>[2x]ASSVEYDDSV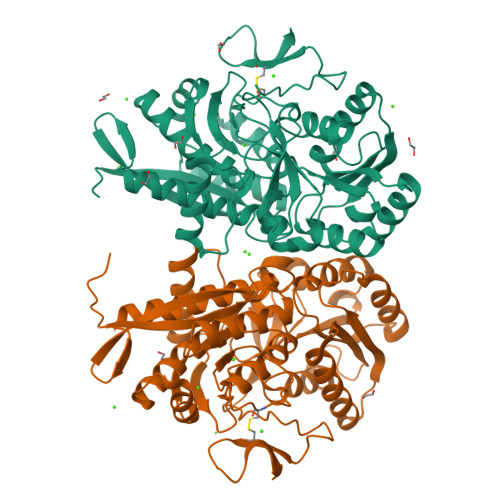TVGILHSLTGTMAISESTLVDTEKMAIDEINAAGGVEVDGKKYKIEYIVEDGASDWPTFAEKSKKLIDQDKVPVVFGGWTSASRKAMLPVYESKEAFLYYPIQYEGQECSKNIFYTGATPNQQSEPATSYMFEKSPAAGKPFYLVGSDYVFPRTSNTITKEQVKSLGGEVVGEDYLPLGNTEVAPIIAKIKAALPDGGVIINTLNGDQNVAFFKQIQDAGITPENGYYVMSYSIAEEEISTIGPEFLEGHYGAWNYMMSIDTPASKKFAADFKAKYGDDRVVADPQESAYNMVYLWKKAVEKAGTFDDDKVREALIGIKFDAPQGPIEVRPNHHISQIVRIGEITSDGQFKIVEESDYPIDPQTWNQFEPTSKGFACDWSDPSKGEKYKL> GPL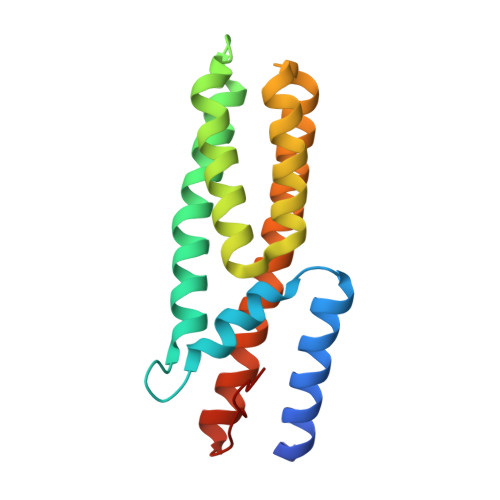GSMDLVQKQKSLQDYTKSLFLEGILDSQFLQLQQLQDESNPDFVSQVVTLFFQDSDRILNDLSLSLDQQVVDFKKVDPHVHQLKGSSSSIGAQRVKNACVVFRSFCEQQNVEACHRCLQQVKQEYYLVKNRLETLFKLEQQIVASGGMIPAVELGF> SNAMKISDAVVSAHIDDEVVLLHLQTGTYFGLDAVGSRIWSLLEEGKRPEEIVDAICAEYSVDRPTV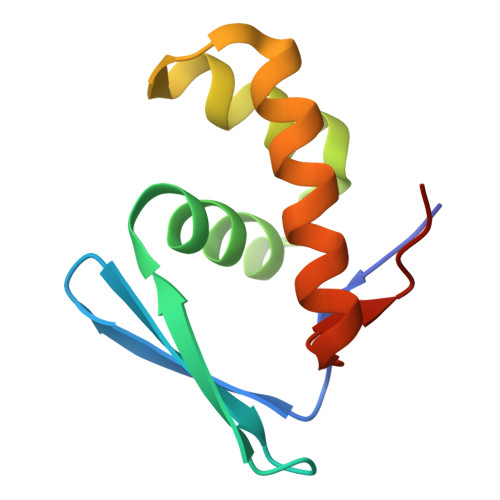ERDLRDFLRALANKELLEGYADEA>MTT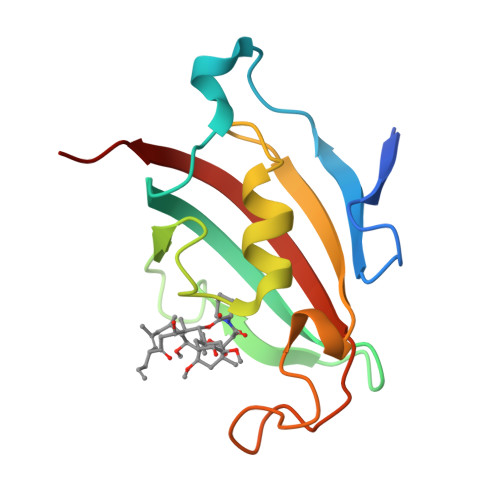EQEFEKVELTADGGVIKTILKKGDEGEENIPKKGNEVTVHYVGKLESTGKVFDSSFDRNVPFKFHLEQGEVIKGWDICVSSMRKNEKCLVRIESMYGYGDEGCGESIPGNSVLLFEIELLSFRELE[2x]>[4x]GAMDIVVNDDLSCRFLEGFNTRDALCKKISMNTCDEGDPFFVADLGDIVRKHETWKKCLPRVTPFYAVKCNDDWRVLGTLAALGTGFDCASNTEIQRVRGIGVPPEKIIYANPCKQISHIRYARDSGVDVMTFDCVDELEKVAKTHPKAKMVLRISTD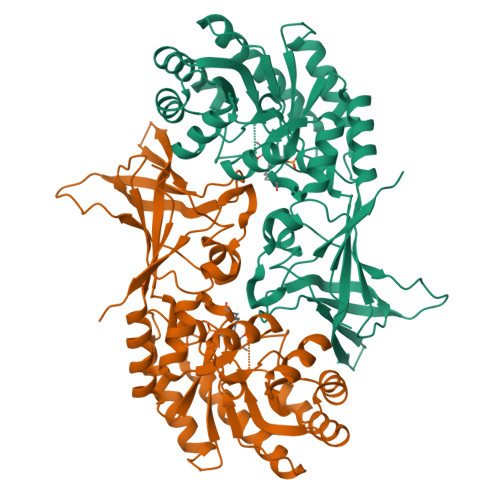DSLARCRLSVKFGAKVEDCRFILEQAKKLNIDVTGVSFHVGSGSTDASTFAQAISDSRFVFDMGTELGFNMHILDIGGGFPGTRDAPLKFEEIAGVINNALEKHFPPDLKLTIVAEPGRYYVASAFTLAVNVIAKKVTPGVQTDVGAHAESNAQSFMYYVNDGVYGSFNCILYDHAVVRPLPQREPIPNEKLYPSSVWGPTCDGLDQIVERYYLPEMQVGEWLLFEDMGAYTVVGTSSFNGFQSPTIYYVVSGLPDHVVRELKSQKS beta-L-arabinofuranose | C5 H10 O5 | 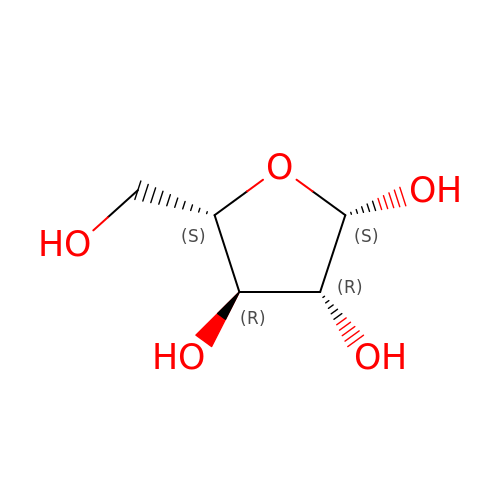HMFHBZSHGGEWLO-KLVWXMOXSA-N8-METHYLNONANOIC ACID | 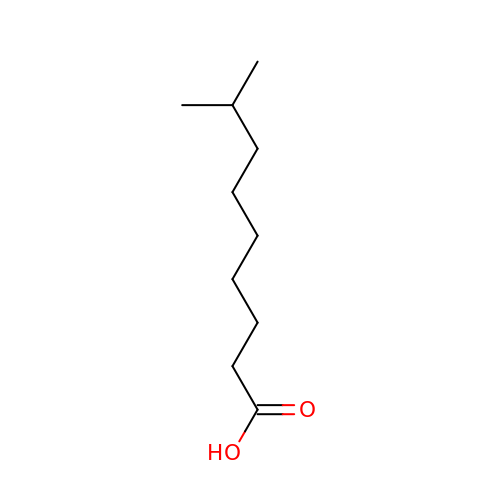C10 H20 O2 | OAOABCKPVCUNKO-UHFFFAOYSA-N>MVKAAAAAASAPTGPGIYSATYSGIPVYEYQFGLKEHVMRRRVDDWINATHILKAAGFDKPARTRILEREVQKDQHEKVQGGYGKYQGTWIPLEAGEALAHRNNIFDRLRPIFEFSPGPDSPPPAPRHTSKPKQPK[2x]

The four DNA binding proteins, MBP1, Swi4, Res1 and Res2 all have the same arrangement of domains, each consisting of an N-terminal DNA binding domain (DBD), a C-terminal heteromerization domain and a central ANK(Ankyrin) repeat region. Swi4 binds to the SCB (Swi6/4 dependent cell cycle box) motif, 5′-CACGAAA-3′, while MBP1, Res1 and Res2 binding to the MCB (Mlu I cell cycle box) sequences with consensus 5′-ACGCGTNA-3′. To clarify whether the DNA binding mode of MBP1 and its orthologues is similar to previously characterized wHTH domain, we have determined the crystal structure of the DBD of PCG2, the orthologue of MBP1 in the rice blast fungus Magnaporthe oryzae, bound to an MCB–DNA motif. Taken together, our data reveal that the MBP1 homologue PCG2 utilizes a novel DNA-binding mode that is distinct from those identified in other proteins with wHTH domain.

The asymmetric unit contains two protein molecules (monomer A and B) and one double-stranded (ds) DNA molecule (14bp, strands C and D). Monomer A and B have a virtually identical conformation with an RMS derivation of only 0.7 Å for their main chains. Both of them comprise a discontinuous, anti-parallel β-barrel structure (β1–6) packed against a loosely associated bundle of four α helices (A–D) with the topology of secondary structures elements arranged in the order β1-β2-β3-β4-αA-αB-β5-β6-αC-αD. In monomer B, the C-terminus was turned towards the N-terminus and located close to the DNA binding site, whereas the residues from 121–128 in monomer A were located further from the DNA binding site. In the complex, the MCB–DNA adopts a right-handed B-DNA. However, in the MCB–DNA as compared with the ideal B-DNA, major groove is narrower and the minor groove wider. The structure reveals that the wing (80-loop), helix B, the 20-loop and helix A are important for MCB–DNA binding and notably, that the wing and helix B recognize the minor groove and major groove of the DNA respectively. The conserved Glu-X-Gly-X-Gly-X-X-Glu (QXGXGXXQ) motif in the 80-loop is located in the minor groove of DNA and contains the residues that make the majority of protein-base interactions with the MCB–DNA. Three types of interactions are observed in this interface. These include the side chain of Q89 that makes hydrogen bonds with the N2 and N3 of dG3 and the side chain of Q82 that is hydrogen bonded to the O2 of dC4 and the N3 of dG5. In contrast with most wHTH structures, helix B is not the main mediator of DNA binding with only two residues (K62 and R65) making contacts with a base and a phosphate of the MCB–DNA. Interface-1, formed in complex A, comprises a larger buried area than interface-2 in complex B (1729.4 Å2 versus 1330.0 Å2) and contains many more hydrogen bonds (26 versus 8) suggesting that there is a greater degree of specificity and affinity in the monomer-A interaction over the monomer-B interaction with DNA.>[2x]MVPDRREQSKAKERLLEREEALAKHMSEREKRPPPKIDPPPSPKAPEPSKRVLKEKQAPLFVDTAVEGTLPPLSLLDPAEVKQKSYSPESLEAMSRLLEIKLKEFGVEVSVDSVHPGPVITRFEIQPAAGVKVSRISNLAKDLARSLAVISVRVVEVIPGKTTVGIEIPNEDRQMVRFSEVLSSPEYDEHKSTVPLALGHDIGGRPIITDLAKMPHLLVAGTTGSGKSVGVNAMLLSILFKSTPSEAR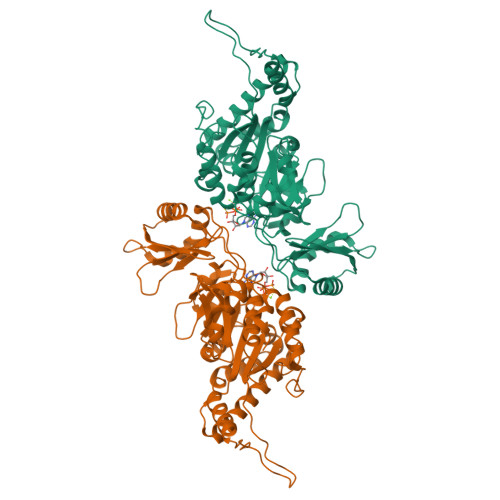LIMIDPKMLELSIYEGIPHLLCPVVTDMKEAANALRWSVAEMERRYRLMAAMGVRNLAGFNRKVKDAEEAGTPLTDPLFRRESPDDEPPQLSTLPTIVVVVDEFADMMMIVGKKVEELIARIAQKARAAGIHLILATQRPSVDVITGLIKANIPTRIAFQVSSKIDSRTILDQGGAEQLLGHGDMLYLPPGTGLPIRVHGAFVSDDEVHRVVEAWKLRGAPDYIEDILAGVDEGGGGGGSFDGGDGSGEGSEDDPLYDEAVRFVTESRRASISAVQRKLKIGYNRAARMIEAMEMAGVVTPMNTNGSREVIAPAPVRDKLHHHHHH The core of the glideosome consists of an atypical class XIV myosin A (PfMyoA) and a divergent actin (PfAct1). PfMyoA is a short myosin with a conserved globular motor domain and a lever arm that binds two light chains: an essential light chain (PfELC) and myosin tail interacting protein (MTIP). PfMyoA is a critical molecule in the parasite life-cycle because it powers the fast motility (~2 µm.s−1) required during motile sporozoite stages, and is essential for providing the force (up to 40 pN) needed for non-motile merozoites to invade erythrocytes. Here, we present the X-ray structures of full-length (FL) PfMyoA complexed to PfELC and MTIP in two states of the motor cycle.

To investigate the structural consequences of the deletion of the N-terminal extension (N-ter) of the PfMyoA heavy chain (HC), we also crystallized the truncated construct (PfMyoA-ΔNter/PfELC/MTIP-Δn). The structure was solved in the post-rigor (PR) state at 3.3 Å resolution (PfMyoA•ΔNter-PR). In all the constructs, MTIP was truncated and lacking the N-terminal extension (residues 1–60) because this extension is predicted to be intrinsically disordered. The similarity of the ΔNter heavy chain and WT PfMyoA structures (rmsd of 0.415 Å on 993 atoms) strongly argues that the dramatic kinetic differences observed between these two constructs are due to an altered equilibrium between the states of the motor cycle. Deletion of the Nter enhanced the duty-ratio (time spent strongly bound to actin) by greatly slowing ADP release to the extent that it rate-limited the overall ATPase cycle, which is ~14 fold slower than WT. Major differences are located at the ELC/converter interface when the PR and the PPS are compared, predominantly due to a sharp kink in the pliant region observed in the PR structures that promotes contacts between the ELC and the motor domain. SAXS experiments demonstrate that this ‘folded-back’ position of the lever arm is not primarily populated in solution and is selected by crystal contacts.

> MAVTNEEIKTASKIVRRVSNVEAFDKSGSVFKGYQIWTDISPTIENDPNIMFVKCVVQQGSKKEKLTVVQIDPPGTGTPYDIDPTHAWNCNSQVDPMSFGDIGLLNHTNIPCVLDFLKHRYLKNQIYTTAVPLIVAINPYKDLGNTTNEWIRRYRDTADHTKLPPHVFTCAREALSNLHGVNKSQTIIVSGESGAGKTEATKQIMRYFASSKSGNMDLRIQTAIMAANPVLEAFGNAKTIRNNNSSRFGRFMQLVISHEGGIRYGSVVAFLLEKSRIITQDDNERSYHIFYQFLKGANSTMKSKFGLKGVTEYKLLNPNSTEVSGVDDVKDFEEVIESLKNMELSESDIEVIFSIVAGILTLGNVRLIEKQEAGLSDAAAIMDEDMGVFNKACELMYLDPELIKREILIKVTVAGGTKIEGRWNKNDAEVLKSSLCKAMYEKLFLWIIRHLNSRIEPEGGFKTFMGMLDIFGFEVFKNNSLEQLFINITNEMLQKNFVDIVFERESKLYKDEGISTAELKYTSNKEVINVLCEKGKSVLSYLEDQCLAPGGTDEKFVSSCATNLKENNKFTPAKVASNKNFIIQHTIGPIQYCAESFLLKNKDVLRGDLVEVIKDSPNPIVQQLFEGQVIEKGKIAKGSLIGSQFLNQLTSLMNLINSTEPHFIRCIKPNENKKPLEWCEPKILIQLHALSILEALVLRQLGYSYRRTFEEFLYQYKFVDIAAAEDSSVENQNKCVNILKLSGLSESMYKIGKSMVFLKQEGAKILTKIQREKLVEWENCVSVIEAAILKHKYKQKVNKNIPSLLRVQAHIRKKMVAQ;> MKQECNVCYFNLPDPESTLGPYDNELNYFTWGPGFEYEPEPQRKPLSIEESFENSEESEESVADIQQLEEKVDESDVRIYFNEKSSGGKISIDNASYNARKLGLAPSSIDEKKIKELYGDNLTYEQYLEYLSICVHDKDNVEELIKMFAHFDNNCTGYLTKSQMKNILTTWGDALTDQEAIDALNAFSSEDNIDYKLFCEDILQ;> MASDMEEKFREAFILFSSCSDHIEMYKFFELMNSFGIILTNDEKAALPNDINMDYWLNFAKKHYNYEQPFKHINNVNEQNTNVQIKIDNFLGIMKALDTRLTESDLNILLQITNPENKSTLNLKTVSQKLTESI> MKRGFARPTPEKPPVIKPENIVLSTPLSIPPPEGKPWWLIVVGVVVVGLLGGMVAMVFASGSHVFGGIGSIFPLFMMVGIMMMMFRGMGGGQQQMSRPKLDAMRAQFMLMLDMLRETAQESADSMDANYRWFHPAPNTLAAAVGSPRMWERKPDGKDLNFGVVRVGVGMTRPEVTWGEPQNMPTDIELEPVTGKALQEFGRYQSVVYNLPKMVSLLVEPWYALVGEREQVLGLMRAIICQLAFSHGPDHVQMIVVSSDLDQWDWVKWLPHFGDSRRHDAAGNARMVYTSVREFAAEQAELFAGRGSFTPRHASSSAQTPTPHTVIIADVDDPQWEYVISAEGVDGVTFFDLTGSSMWTDIPERKLQFDKTGVIEALPRDRDTWMVIDDKAWFFALTDQVSIAEAEEFAQKLAQWRLAEAYEEIGQRVAHIGARDILSYYGIDDPGNIDFDSLWASRTDTMGRSRLRAPFGNRSDNGELLFLDMKSLDEGGDG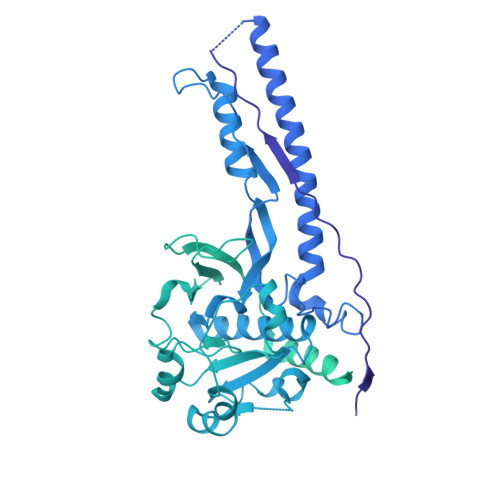PHGVMSGTTGSGKSTLVRTVIESLMLSHPPEELQFVLADLKGGSAVKPFAGVPHVSRIITDLEEDQALMERFLDALWGEIARRKAICDSAGVDDAKEYNSVRARMRARGQDMAPLPMLVVVIDEFYEWFRIMPTAVDVLDSIGRQGRAYWIHLMMASQTIESRAEKLMENMGYRLVLKARTAGAAQAAGVPNAVNLPAQAGLGYFRKSLEDIIRFQAEFLWRDYFQPGVSIDGEEAPALVHSIDYIRPQLFTNSFTPLEVSVGGPDIEPVVAQPNGEVLESDDIEGGEDEDEEGVRTPKVGTVIIDQLRKIKFEPYRLWQPPLTQPVAIDDLVNRFLGRPWHKEYGSACNLVFPIGIIDRPYKHDQPPWTVDTSGPGANVLILGAGGSGKTTALQTLICSAALTHTPQQVQFYCLAYSSTALTTVSRIPHVGEVAGPTDPYGVRRTVAELLALVRERKRSFLECGIASMEMFRRRKFGGEAGPVPDDGFGDVYLVIDNYRALAEENEVLIEQVNVIINQGPSFGVHVVVTADRESELRPPVRSGFGSRIELRLAAVEDAKLVRSRFAKDVPVKPGRGMVAVNYVRLDSDPQAGLHTLVARPALGSTPDNVFECDSVVAAVSRLTSAQAPPVRRLPARFGVEQVRELASRDTRQGVGAGGIAWAISELDLAPVYLNFAENSHLMVTGRRECGRTTTLATIMSEIGRLYAPGASSAPPPAPGRPSAQVWLVDPRRQLLTALGSDYVERFAYNLDGVVAMMGELAAALAGREPPPGLSAEELLSRSWWSGPEIFLIVDDIQQLPPGFDSPLHKAVPFVNRAADVGLHVIVTRTFGGWSSAGSDPMLRALHQANAPLLVMDADPDEGFIRGKMKGGPLPRGRGLLMAEDTGVFVQVAATEVRR>[18x]FTLIELMIVVAIIGILAAIAIPNFIKFQARSKQSEAKTNLKALYTAQKSFFSEKDRYSDFANEIGFAPERGNRYGYRVSAAAGDCEVRNAADLPVPAAGVPCISND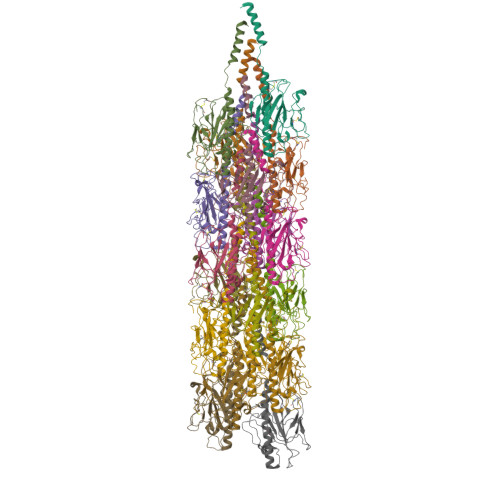SFRFGANSAIDDPTPVVARFVPQGAAGWNTTLGVQPTIADCPNCNFFAGARGNADNEATFDDWVIAGFEGSGQVGPCSEAGNVASGTPYNTRNDVACDGAAQ>[2x]SKNGLKKRKLTNPVQLDDFDGYIKDMAKDSDYKFSLQFEELK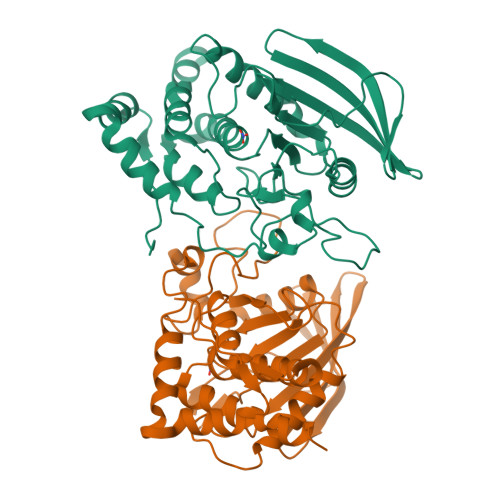LIGLDIPHFAADLPMNRCKNRYTNILPYDFSRVRLVSMNEEEGSDYINANYIPGYNSPQEYIATQGPLPETRNDFWKMVLQQKSQIIVMLTQCNEKRRVKCDHYWPFTEDPIAYGDITVEMLSEEEHTDWVYRNFRISYADEVQDVMHFNYTAWPDHGVPTANAAESILQFVQMVRQKSVKSKGPMIIHCSAGVGRTGTFIALDWLLQHIRDHEFVDILGLVSDMRSYRMSMVQTEEQYIFIHQCVQLMWQKKKQQFCISDVIYENVSKS>[6x]GSMDLKTAVFNAARDGKLR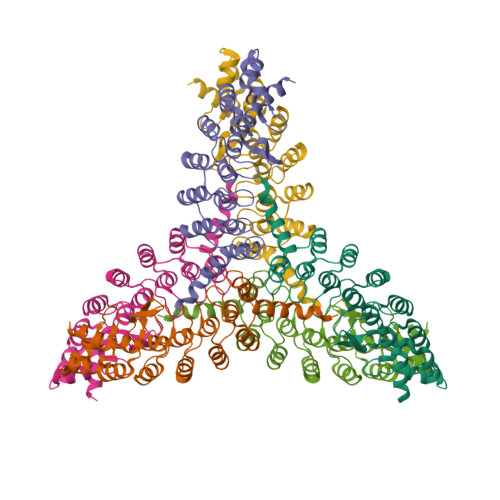LLTKLLASKSKEEVSSLISEKTNGATPLLMAARYGHLDMVEFLLEQCSASIEVGGSVNFDGETIEGAPPLWAASAAGHLKVVQSLLNHGASVNNTTLTNSTPLRAACFDGHLEIVKYLVEHKADLEVSNRHGHTCLMISCYKGHKEIAQYLLEKGADVNRKSVKGNTALHDCAESGSLDIMKMLLMYCAKMEKDGYGMTPLLSASVTGHTNIVDFLTHHAQTSKTER(2R)-2-hydroxy-2-{2-[4-(3-hydroxy-9,10-dioxo-9,10-dihydroanthracene-2-sulfonyl)piperazin-1-yl]-2-oxoethyl}butanedioic 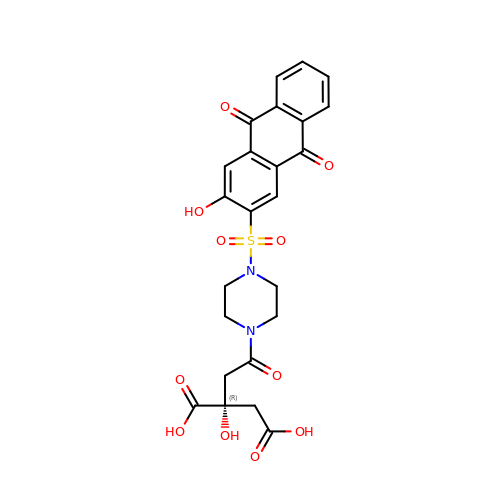acid | C24 H22 N2 O11 S | BDGXYHKLUUUHLU-XMMPIXPASA-N> LGTNYLLSGQTLDREGHLKNGDFDLVMQDDCNLVLYNGNWQSNTA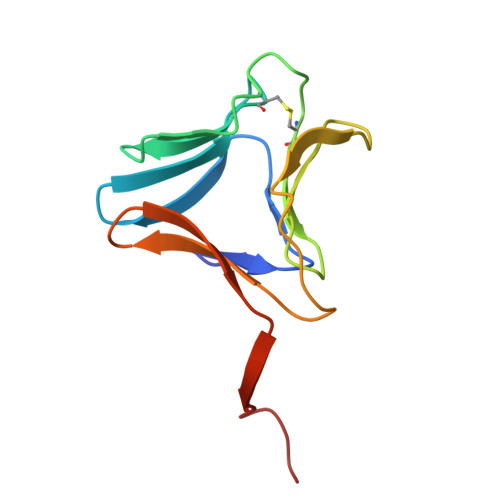NKGRDCKLTLTDYGELVIKNGDGSTVWRSRAQSVKGNYAAVVHPDGRLVVFGPSVFKIDPWVPG>[4x]CTTPTAVAVTFDLTATTTYGENIYLVGSISQLGDWETSDGIALSAD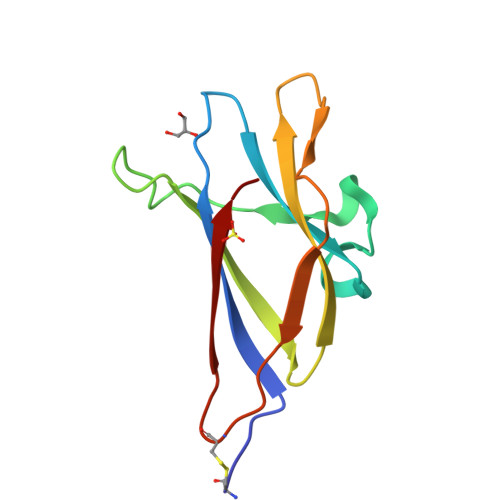KYTSSDPLWYVTVTLPAGESFEYKFIRIESDDSVEWESDPNREYTVPQACGTSTATVTDTWR>[6x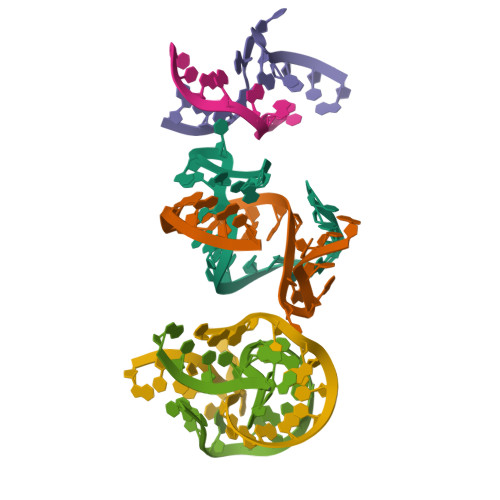]GUCUAUGAAGGCUGGAGAC>TDLISPVVLTNYLNSQYYGEIGIGT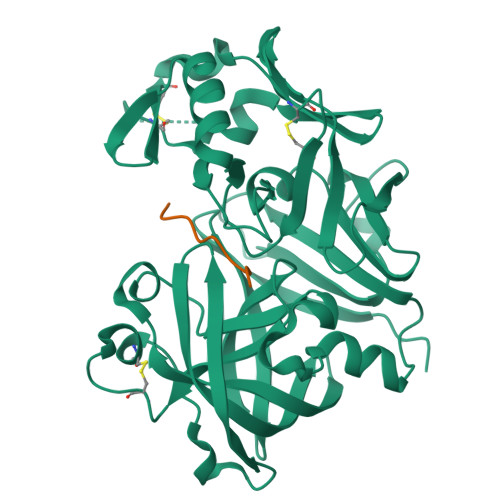PPQTFKVIFDTGSANLWVPSTKCSRLYLACGIHSLYESSDSSSYMENGDDFTIHYGSGRVKGFLSQDSVTVGGITVTQTFGEVTQLPLIPFMLAQFDGVLGMGFPAQAVGGVTPVFDHILSQGVLKEKVFSVYYNRGPHLLGGEVVLGGSDPQHYQGDFHYVSLSKTDSWQITMKGVSVGSSTLLCEEGCEVVVDTGSSFISAPTSSLKLIMQALGAKEKRLHEYVVSCSQVPTLPDISFNLGGRAYTLSSTDYVLQYPNRRDKLCTVALHAMDIPPPTGPVWVLGATFIRKFYTEFDRHNNRIGFALAR[4x]> MHHHHHHEFMQKIGILGAMREEITPILELFGVDFEEIPLGGNVFHKGVYHNKEIIVAYSKIGKVHSTLTTTSMILAFGVQKVLFSGVAGSLVKDLKIN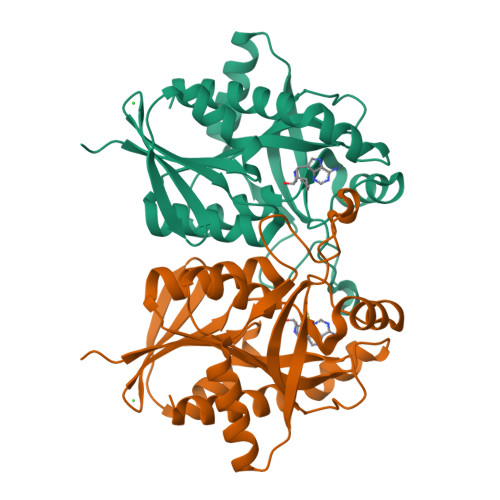DLLVATQLVQHDVDLSAFDHPLGFIPESAIFIETSGSLNALAKKIANEQHIALKEGVIASGDQFVHSKERKEFLVSEFKASAVEMEGASVAFVCQKFGVPCCVLRSISDNADEKAGMSFDEFLEKSAHTSAKFLKSMVDEL>GPLGSRPFRFSPEPTLEDIRRLHAEFAAERDWEQFHQPRNLLLALVGEVGELAELFQWKSDTEPGPQAWPPKERAALQEELSDVLIYLVALAARCHVDLPQAVISK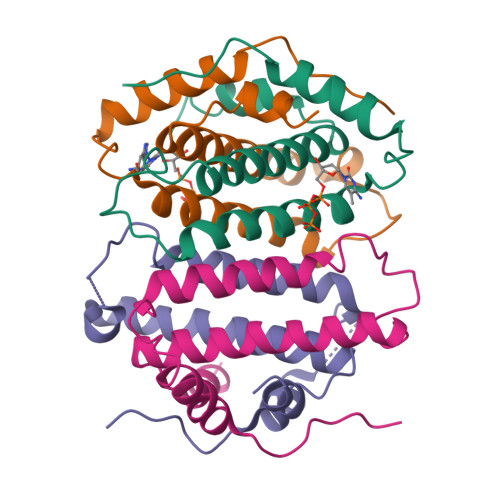MDTNR[4x]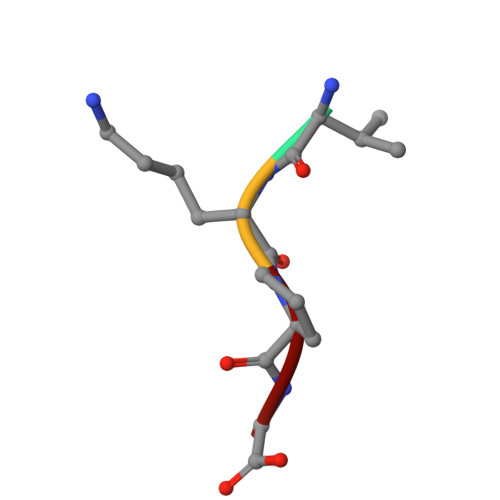> VKPG>YLSIAFPENTKLDWKPVTKNTRYCPMGGEWFLEPGLQEESFLSSTPIGATPSKSDGFLCHAAKWVTTCDFRWYGPKYITHSIHNIKPTRSDCDTALASYKSGTLVSLGFPPESCGYASVTDSEFLVIMITPHHVGVDDYRGHWVDPLFVGGECDQSYCDTIHNSSVWIPADQTKKNICGQSFTPLTVTVAYDKTKEIAAGGIVF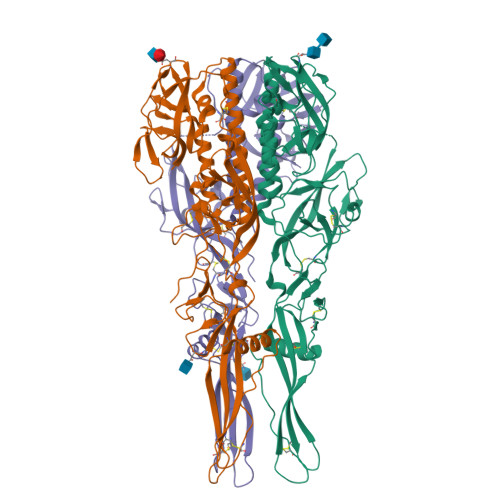KSKYHSHMEGARTCRLSYCGRNGIKFPNGEWVSLDVKTRIQEKHLLPLFKECPAGTEVRSTLQSDGAQVLTSEIQRILDYSLCQNTWDKVERKEPLSPLDLSYLASKSPGKGLAYTVINGTLSFAHTRYVRMWIDGPVLKEPKGKRESPSGISSDIWTQWFKYGDMEIGPNGLLKTAGGYKFPWHLIGMGIVDNELHELSEANPLDHPQLPHAQS[3x]>MSVLFISDLNLEAERPDITRAFLSFLDERARRAEALYILGDFFEAWIGDDGMDAFQRSIAQSLRQVADGGTRIYLMHGNRDFLIGKAFCREAGCTLLPDPSVIDLYGEPVLLMHGDSLCTRDEAYMRLRRWLRNPLTLWVLRHLPLATRHKLARKLRKESRAQTRMKAVDIIDVTPEEVPRVMRGHGVRTLIHGHTHRPAEHPLDIDGQPARRIVLGDWDRQGWALEIDANGHRQAPFPLLEHHHHHH[2x]

In the fourth step in this pathway, UDP-2,3-diacylglucosamine is hydrolyzed to 2,3-diacylglucosamine-1-phosphate (also called lipid X) and UMP. This step is catalyzed by the specific pyrophosphatase LpxH in 70% of gram-negative bacteria, including E. coli and Pseudomonas aeruginosa, and by LpxI in the remaining 30%345. LpxH shares sequence similarity with metallophosphoesterases and requires Mn2+ ions for phosphatase activity. PaLpxH consists of two domains: a catalytic domain homologous to metallophosphoesterases (MPEs) and a helical insertion domain (HI domain) inserted in the middle of the catalytic domain.

To investigate enzymatic reaction mechanism, a mutant was prepared in which Mn1-coordinated His10 was replaced with Asn (H10N). Its structure was determined with (Mn2 bound form) and without (Mn2 unbound form) manganese ion. As expected, the H10N mutant did not bind to Mn1. Although it was prepared using the same protocol as the wild type, this PaLpxH mutant did not capture a product molecule (lipid X). The substrate molecule UDP-2,3-diacylglucosamine was also not observed in the electron density map. However, except for the loss of Mn1, no large conformational change occurred in the vicinity of the mutated Asn10 residue, and the structure of the whole catalytic domain was similar to that of the wild type. There is no electron density for the C-terminal half of α6 and the following loop region (residues 161–169 in P212121 crystal with one Mn2+, 159–165 in P212121 crystal with no Mn2+) in the apo form, indicating they are highly mobile and disordered. In the apo form, α7 (residues 169–172) disappears and a loop (P212121 with one Mn2+) or a short 310 helix at residues 168–170 (P212121 with no Mn2+) is created. A significant structural change in residues 158–172 is important for the recognition of lipid X (and probably also the substrate); the binding site is wide open in the apo form, whereas in the EP complex, two alpha helices (α6 and α7) are formed to assemble a stable EP complex.>MIAAQLLAYYFTELKDDQVKKIDKYLYAMRLSDETLIDIMTRFRKEMKNGLSRDFNPTATVKMLPTFVRSIPDGSEKGDFIALDLGGSSFRILRVQVNHEKNQNVHMESEVYDTPENIVHGSGSQLFDHVAECLGDFMEKRKIKDKKLPVGFTFSFPCQQSKIDEAILITWTKRFKASGVEGADVVKLLNKAIKKRGDYDANIVAVVNDTVGTMMTCGYDDQHCEVGLIIGTGTNACYMEELRHIDLVEGDEGRMCINTEWGAFGDDGSLEDIRTEFDREIDRGSLNPGKQLFEKMVSGMYLGELVRLILVKMAKEGLLFEGRITPELLTRGKFNTSDVSAIEKNKEGLHNAKEILTRLGVEPSDDDCVSVQHVCTIVSFRSANLVAATLGAILNRLRDNKGTPRLRTTVGVNGSLYKTHPQYSRRFHKTLRRLVPDSDVRFLLSESGSGKGAAMVTAVAYRLAEQHRQIEETLAHFHLTKDMLLEVKKRMRAEMELGLRKQTHNNAVVKMLPSFVRRTPDGTENGDFLALDLGGTNFRVLLVKIRSGKKRTVEMHNKI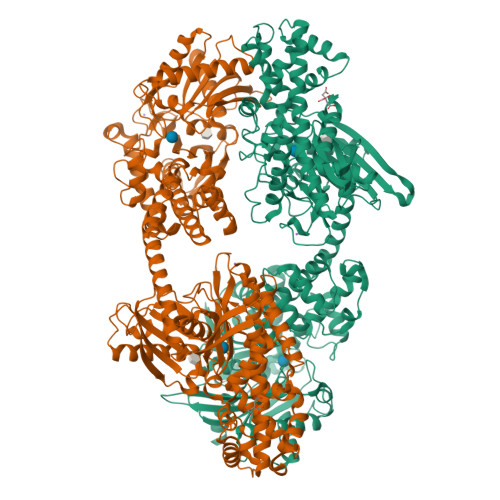YAIPIEIMQGTGEELFDHIVSCISDFLDYMGIKGPRMPLGFTFSFPCQQTSLDAGILITWTKGFKATDCVGHDVVTLLRDAIKRREEFDLDVVAVVNDTVGTMMTCAYEEPTCEVGLIVGTGSNACYMEEMKNVEMVEGDQGQMCINMEWGAFGDNGCLDDIRTHYDRLVDEYSLNAGKQRYEKMISGMYLGEIVRNILIDFTKKGFLFRGQISETLKTRGIFETKFLSQIESDRLALLQVRAILQQLGLNSTCDDSILVKTVCGVVSRRAAQLCGAGMAAVVDKIRENRGLDRLNVTVGVDGTLYKLHPHFSRIMHQTVKELSPKCNVSFLLSEDGSGKGAALITAVGVRLRTEASS[2x]>AELLLGVNIDHIATLRNARGTAYPDPVQAAFIAEQAGADGITVHLREDRRHITDRDVRILRQTLDTRMNLEMAVTEEMLAIAVETKPHFCCLVPEKRQEVTTEGGLDVAGQRDKMRDACKRLADAGIQVSLFIDADEEQIKAAAEVGAPFIEIHTGCYADAKTDAEQAQELARIAKAATFAASLGLKVNAGHGLTYHNVKAIAAIPEMHELNIGHAIIG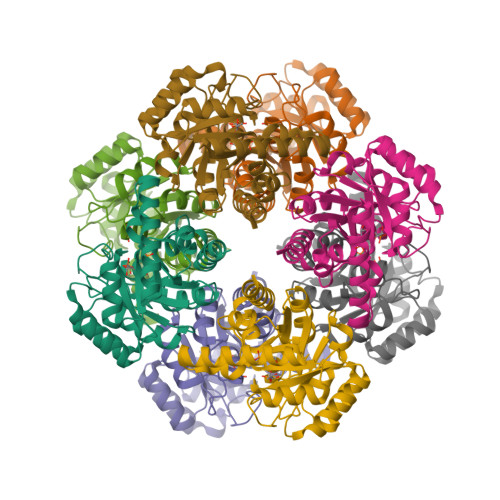RAVMTGLKDAVAEMKRLMLEARG[4x]> MADDQGCIEEQGVEDSANEDSVDAKPDRSSFVPSLFSK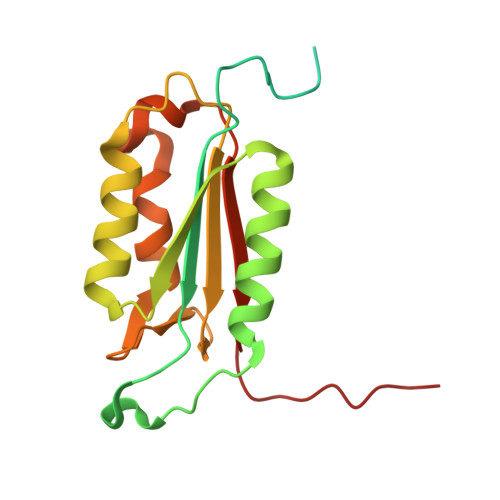KKKNVTMRSIKTTRDRVPTYQYNMNFEKLGKCIIINNKNFDKVTGMGVRNGTDKDAEALFKCFRSLGFDVIVYNDCSCAKMQDLLKKASEEDHTNAACFACILLSHGEENVIYGKDGVTPIKDLTAHFRGDRCKTLLEKPKLFFIQACRGTELDDGIQAD> MKQIKLLFLLASASVTGAFAQSNGLTDMSQSRYAKMANTGIDAVHWTNGFWGERFNVFSGTSLQSMWNTWNTPEVSHGFRNFEIAAGVCKGEHWGPPFHDGDMYKWMEGVASVYAVNKDPELDKLMDNFIACVVKAQRADGYIHTPVVIEELNKGIDSHTLADSQQQTVIGTKVGSEDEKGAFANRLNFETYNLGHLMMAGIVHHRATGKTTLFDAA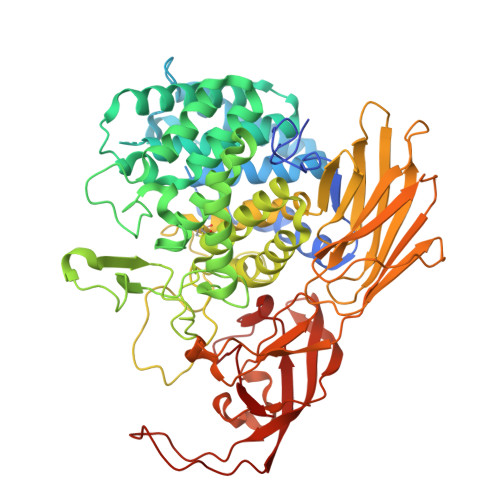VKATDFLCHFYETASAELARNAICPSHYMGVVEMYRATGNPRYLELSKNLIDIRGMVESGTDDNQDRIPFRDQYRAMGHAVRANYLYAGVADVYAETGEQQLMKNLTSIWNDIVTRKMYVTGACGALYDGTSPDGTCYEPDSIQKVHQSYGRPYQLPNSTAHNETCANIGNMLFNWRMLEVTGDAKYAELVETCLYNSVLSGISLDGKKYFYTNPLRISADLPYTLRWPKERTEYISCFCCPPNTLRTLCQAQNYAYTLSPEGIYCNLYGANTLTTNWKDKGELALVQETDYPWEGNVRVTLNKVPRKAGAFSLFFRIPEWCGKAALTVNGQPVSMNAKANTYAEVNRTWKKGDVVELVMDMPVCLLEAHPLAEEIRNQVVVKRGPLVYCLESMDIANGEKIDNILIPADIKLIPKKTTIEGSSIVALEGKARLASSESWEGVLYRPVVQAEKTVDIRLIPYYAWGNRGKGEMTVWMPLAR>[2x]DWPVYHRIDGPIVMIGFGSIGRGTLPLIERHFAFDRSKLVVIDPSDEARKLAEARGVRFIQQAVTRDNYRELLVPLLTAGPGQGFCVNLSVDTSSLDIMELARENGALYIDTVVEPWLGFYFDPDLKPEARSNYALRETVLAARRNKPGGTTAVSCCGANPGMVSWFVKQA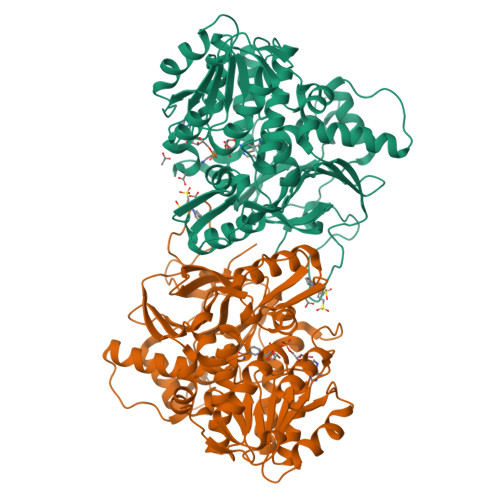LVNLAADLGVTGEEPTTREEWARLAMDLGVKGIHIAERDTQRASFPKPFDVFVNTWSVEGFVSEGLQPAELGWGTFERWMPDNARGHDSGCGAGIYLLQPGANTRVRSWTPTAMAQYGFLVTHNESISIADFLTVRDAAGQAVYRPTCHYAYHPCNDAVLSLHEMFGSGKRQSDWRILDETEIVDGIDELGVLLYGHGKNAYWYGSQLSIEETRRIAPDQNATGLQVSSAVLAGMVWALENPNAGIVEADDLDFRRCLEVQTPYLGPVVGVYTDWTPLAGRPGLFPEDIDTSDPWQFRNVLVRD>SGGGDGSTYSAEIRRTTMGVPHIKAGNWGSAGYGFGYVQAQDNLCTMADSFLTYRGERSRHLGGSAQLVYNSTLGRPRNIDSDFFHRHVISDEAVDRTMAAQPAKLLQMVEGFAAGYNRYVREAKAGGSAHAACRSEAWVQPITARDVWRRIYAANLAGGYSNFAEAIANAQPPQAKA[4x];>GAQEPAAFEPGRTRAPSLQVGGELGVG[4x];>[4x]SNMYGFGTAATGEGSGVLFGNPHWYWKGPDRFYQAQLTIDGEANVSGVSFLGLPVIQIGFNDSVAWSHTVSTARRFGFFQLSLVQGEPTSYLRDGVPVKMKPATITVPSRNADGSVSDVTRTLYHSEFGPLVNLAGLNPALAWSQGTAFAIRDINGENFRTLRTWMRWNQAKSLDEFIAIQKEEASIPWVNTVAVGRGSAKAWYADIGAVPNVSPAQTAACTTPFGMAVGQALPNVPFFDGSRSECDWLTDADSVQKGAVGVSRMPSLQRDDYVGNMNDSYWLANVHAPLTGYPAIFGPAGTSAQTLRTRMGHTMALERLAGTDGYAGNKATSAVVREMVLGSRVFSAERFKDEVLDLICTPAQWTVNGAAVDAAQACAVLAAWDNRGRKDSRGSHLWDEFWSRVPTASLFTVPFSAADPLNTPRGINAAAADALRQAMATAIARVGQSGYALDAPRGEVLYATRGGTRLPLYGGCGAMGYFTITCSENDITQGGYSMDGQPNASNSYMQVVSFPASGVQAHTFLTFSLSDDPASPHHGDYTKAYSAGQWLRVPFTEAEITGNADYRTATVKELEHHHHHH

The recombinant MacQ protein exhibited bifunctional acylase activity against various ranges of AHLs and against multiple β-lactam antibiotics, including penicillin G, ampicillin, and amoxicillin. The MacQ protein is comprised of 806 amino acid residues, including an N-terminal signal peptide, and belongs to the N-terminal nucleophile (Ntn) hydrolase superfamily. AHL-acylase is one of the enzymes capable of inactivating AHLs via hydrolysis of the amide bond of the acyl side-chain to produce homoserine lactone (HSL) and fatty acid. The MacQ structure clearly revealed a typical Ntn-hydrolase fold comprised of a four-layered α-β-β-α motif45 mainly composed of two polypeptide chains, α- and β-chains, generated by self-cleaving activity.

The crystal structures of MacQ, both ligand-free and in complex with the reaction products of decanoic acid (C10) and phenyl acetic acid (PAA), were determined at 2.6 Å, 2.2 Å, and 1.75 Å resolution, respectively. The C10 complex crystallized in the P1 space group, similar to that of ligand-free MacQ, while the PAA complex crystallized in the P21 space group. The structure of the PAA complex was solved by the molecular replacement method using the ligand-free MacQ as a search model. The asymmetric unit of the P21 lattice also contains two PAA-bound molecules, which superimposed well on those of ligand-free and C10 complexes of MacQ in the P1 lattice, with an RMS difference of ~1.0 Å for 1505 Cα atoms. The reaction product, C10/PAA, was successfully trapped at the hydrophobic active-site pocket, while the electron density for the hydrolyzed counterpart, HSL/6-aminopenicillanic acid (6-APA), was not observed. The results suggest that the more hydrophilic HSL/6-APA diffused into the solvent immediately after the enzymatic amidohydrolyzing reaction. In contrast, PAA was bound in the same state in each active-site pocket without covalent bonds. The atomic models of PAA in two different conformations fit well to the observed electron density and were refined with reasonable B-factor values in all active sites. The C10/PAA was accommodated in the highly hydrophobic active-site pocket created by the side-chains of Trp24β, Phe32β, Phe50β, Gln57β, Ile58β, His68β, Val70β, Trp165β, Trp189β, and Val190β. First, the SP is observed in all heterodimeric units of MacQ in the same conformation, both in the presence and absence of ligands.>SIFKGSGVAIITPFTNTGVDFDKLSELIEWHIKSKTDAIIVCGTTGEATTMTETERKETIKFVIDKVNKRIPVIAGTGSNNTAASIAMSKWAESIGVDGLLVITPYYNKTTQKGLVKHFKAVSDAVSTPIIIYNVPGRTGLNITPGTLKELCEDKNIVAVKEASGNISQIAQIKALCGDKLDIYSGNDDQIIPILALGGIGVISVLANVIPEDVHNMCELYLNGKVNEALKIQLDSLALTNALFIETNPIPVKTAMNLMNMKVGDLRLPLCEMNENNLEILKKELKAYNLM[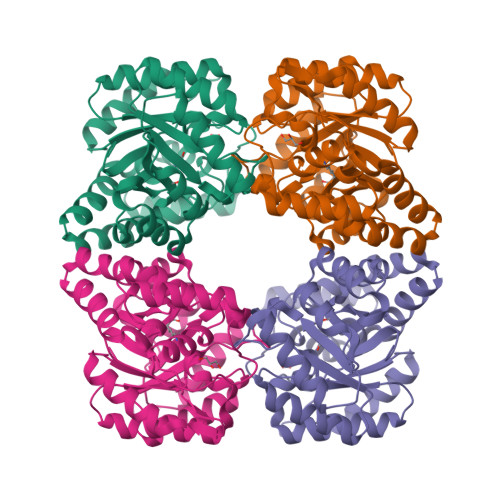2x]>[4x]FARNEKEAKDSAITFIQKSAAIKAGARSAEDIKLDKVNLGGELSGSNMYVYNISTGGFVIVSGDKRSPEILGYSTSGSFDANGKENIASFMESYVEQIKENKKLDTTYAGTAEIKQPVVKSLLDSKGIHYNQGNPYNLLTPVIEKVKPGEQSFVGQHAATGCVATATAQ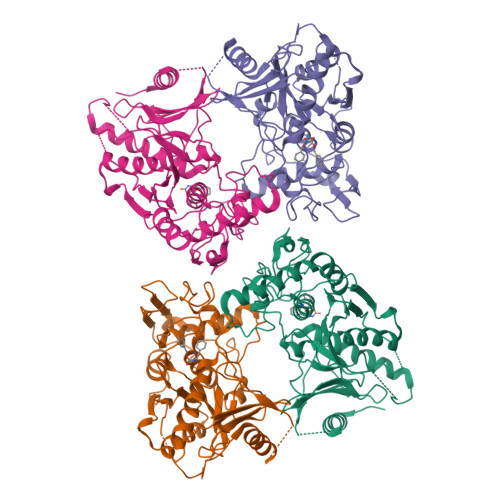IMKYHNYPNKGLKDYTYTLSSNNPYFNHPKNLFAAISTRQYNWNNILPTYSGRESNVQKMAISELMADVGISVDMDYGPSSGSAGSSRVQRALKENFGYNQSVHQINRGDFSKQDWEAQIDKELSQNQPVYYQGVGKVGGHAFVIDGADGRNFYHVNWGWGGVSDGFFRLDALNPSALGTGGGADGFNGYQSAVVGIKP> MHHHHHHTFGNMERDLFEKKFKEIKDKWVTDKQADEFIETADKYADKAVQMSAVASRAEYYRMYVSRKYQYKKEFVEKLKQVYKESGASHVTSKKDLMLAFDDAKRKSTIGRQENGLFVTSFAEDMALLFTDQGKLKSADQIE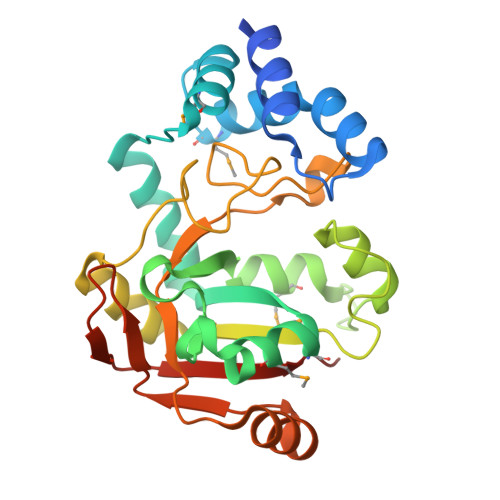NIKGVDSGKYSDGVYQYEYDSELTKNIDKLGYIRTASGDTPGANSLNIPGCQTWSGKHIENSESELIFPSISVKDLKSKAVLAEIDAKGYFEIIDPTIIAPNGDHKKVTGRFKIKKMQDRMQDRK> APTIPQGQGKVTFNNTVVDAPCSISQKSADQSIDFGQLSKSFLEAGGVSKPMDLDIELVNCDITAFKGGNGAKKGTVKLAFT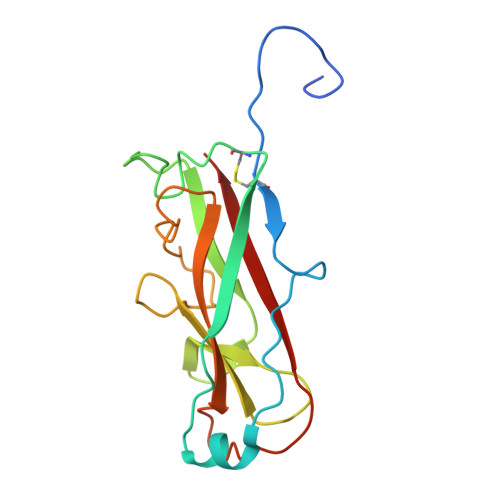GPIVNGHSDELDTNGGTGTAIVVQGAGKNVVFDGSEGDANTLKDGENVLHYTAVVKKSSAVGAAVTEGAFSAVANFNLTYQ>[4x]MSQHNEKNPHQHQSPLHDSSEAKPGMDSLAPEDGSHRPAAEPTPPGAQPTAPGSLKAPDTRNEKLNSLEDVRKGSENYALTTNQGVRIA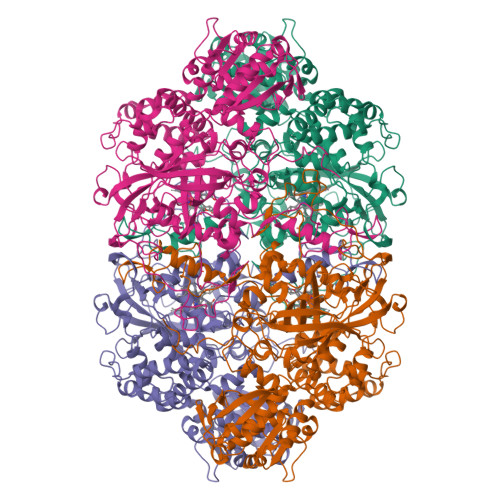DDQNSLRAGSRGPTLLEDFILREKITHFDHERIPERIVHARGSAAHGYFQPYKSLSDITKADFLSDPNKITPVFVRFSTVQGGAGSADTVRDIRGFATKFYTEEGIFDLVGNNTPIFFIQDAHKFPDFVHAVKPEPHWAIPQGQIAHDTFWDYVSLQPETLHNVMWAMSDRGIPRSYRTMEGFGIHTFRLINAEGKATFVRFHWKPLAGKASLVWDEAQKLTGRDPDFHRRELWEAIEAGDFPEYELGFQLIPEEDEFKFDFDLLDPTKLIPEELVPVQRVGKMVLNRNPDNFFAENEQAAFHPGHIVPGLDFTNDPLLQGRLFSYTDTQISRLGGPNFHEIPINRPTCPYHNFQRDGMHRMGIDTNPANYEPNSINDNWPRETPPGPKRGGFESYQERVEGNKVRERSPSFGEYYSHPRLFWLSQTPFEQRHIVDGFSFELSKVVRPYIRERVVDQLAHIDLTLAQAVAKNLGIELTDDQLNITPPPDVNGLKKDPSLSLYAIPDGDVKGRVVAILLNDEVRSADLLAILKALKAKGVHAKLLYSRMGEVTADDGTVLPIAATFAGAPSLTVDAVIVPCGNIADIADNGDANYYLMEAYKHLKPIALAGDARKFKATIKIADQGEEGIVEADSADGSFMDELLTLMAAHRVWSRIPKIDKIPA>MSLLIRGATVVTHEESYRADVLCANGLIQAIGENLETPSGCDVLDGGGQYLMPGGIDPHTHMQLPFMGTVASEDFFSGTAAGLAGGTTSIIDFVIPNPRQSLLEAFHTWRGWAQKSAADYGFHVAITWWSDEVAREMGELVAQHGVNSFKHFMAYKNAIMAADDTLVASFERCLELGAVPTVHAENGELVFHLQQKLLAQGLTGPEAHPLSRPPQVEGEAASRAIRIAETLGTPLYLVHISSREALDEIAYARAKGQPVYGEVLAGHLLLDDSVYRHPDWATAAGYVMSPPFRPVEHQEALWRGLQSGNLHTTATDHCCFCAEQKAMGRDDFSKIPNGTAGIEDRMALLWDAGVNSGRLSMHEFVALTSTNTAKIFNLFPRKGAIRVGADADLVLWDPQGSRTLSAATHHQRVDFNIFEGRTVRGIPSHTISQGKLLWAAGDLRAEPGAGRYVERPAYPSVYEVLG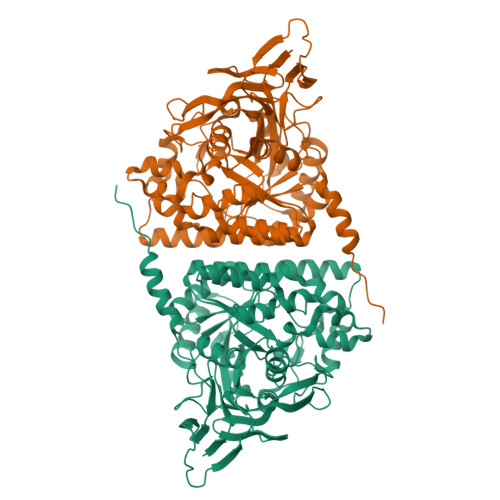RRAERQRPVAVERHHHHHH[2x]> MSFFHGVTVTNVDIGARTIALPASSVIGLCDVFTPGAQASAKPNVPVLLTSKKDAAAAFGIGSSIYLACEAIYNRAQAVIVAVGVETAETPEAQASAVIGGISAAGERTGLQALLDGKSRFNAQPRLLVAPGHSAQQAVATAMDGLAEKLRAIAILDGPNSTDEAAVAYAKNFGSKRLFMVDPGVQVWDSATNAARNAPASAYAAGLFAWTDAEYGFWSSPSNKEIKGVTGTSRPVEFLDGDETCRANLLNNANIATII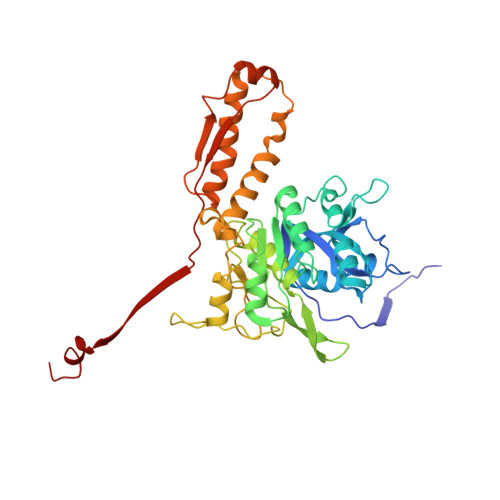RDDGYRLWGNRTLSSDSKWAFVTRVRTMDLVMDAILAGHKWAVDRGITKTYVKDVTEGLRAFMRDLKNQGAVINFEVYADPDLNSASQLAQGKVYWNIRFTDVPPAENPNFRVEVTDQWLTEVLDVA> GSMEPGRGGTETVGKFEFSRKDLIGHGAFAVVFKGRHREKHDLEVAVKCINKKNLAKSQTLLGKEIKILKELKHENIVALYDFQEMANSVYLVMEYCNGGDLADYLHAMRTLSEDTIRLFLQQIAGAMRLLHSKGIIHRDLKPQNILLSNPAGRRANPNSIRVKIADFGFARYLQSNMMAATLCGSPMYMAPEVIMSQHYDGKADLWSIGTIVYQCLTGKAPFQASSPQDLRLFYEKNKTLVPTIPRETSAPLRQLLLALLQRNHKDRMDFDEFFHHPFLDASP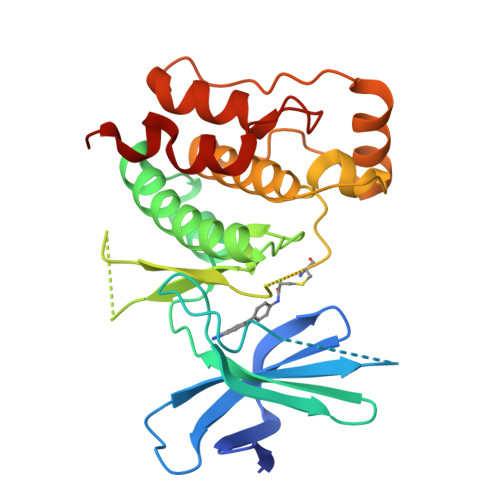S>MKLIIVGAHSSVPSGYGRVMRAIVPRISKAHEVIVFGIHAFGRSVHANIEEFDAQTAEHVRGLNEQGFYYSGLSEFIDVHKPDIVMIYNDPIVIGNYLLAMGKCSHRTKIVLYVDLVSKNIRENLWWIFSHPKVVGVMAMSKCWISDICNYGCKVPINIVSHFVDTKTIYDARKLVGLSEYNDDVLFLNMNRNTARKRLDIYVLAAARFISKYPDAKVRFLCNSHHESKFDLHSIALRELVASGVDNVFTHLNKIMINRTVLTDERVDMMYNACDVIVNCSSGEGFGLCSAEGAVLGKPLIISAVGGADDYFSGDCVYKIKPSAWISVDDRDGIGGIEGIIDVDDLVEAFTFFKDEKN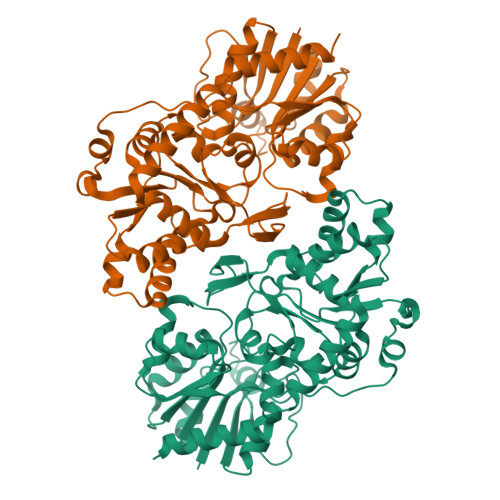RKEYGKRVQDFVKTKPTWDDISSDIIDFFNSLLRVESRETPGNEEHPLEHHHHHH[2x]Here we studied 30 congeneric ligands that each present a distinct heteroarene for stacking between tyrosine residues at the dimer interface of procaspase-6. Complex X-ray crystal structures of 10 analogs showed that stacking geometries were well conserved, while high-accuracy computations showed that heteroarene stacking energy was well correlated with predicted overall ligand binding energies. Here we employed a congeneric set of molecular glues for procaspase-6 to study diverse heteroarene stacking on tyrosine side chains under physiologically relevant conditions. As a model system, this protein–ligand interaction exhibits desirable features such as a shape-persistent binding site, a conserved ligand binding mode across diverse analogs, and the positioning of the probe heteroarene at the terminus of the ligand structure.

To confirm that binding poses and stacking interactions were conserved across analogs 1–30, we solved procaspase-6 complex crystal structures for 10 representative analogs spanning 3 orders of magnitude in measured KD value. Importantly, all 10 structures revealed binding poses almost exactly analogous to that adopted by 1, with the probe heterocycles positioned in apparently productive stacking interactions with tyrosine 198A and 198B. Also consistent with established guidance was the trend of increasing potencies from thiophene to furan, to pyrazole and imidazole (7 and 8) as well as the favorable effect of N-methylation of nitrogen-bearing heterocycles in the context of indazole (cf. 9 vs 15), imidazole (cf. 8 vs 18), and triazole (cf. 22 vs 24). Recently, Bootsma et al. noted the importance in heteroarene stacking of the relative positioning of ring heteroatoms in otherwise similar heterocycles. By contrast, the distal arrangement is favored when the heteroatoms are “dissimilar” (i.e., one is an amine-like nitrogen atom). We evaluated these predictions across the four relevant comparator sets, confining the analysis to analogs bearing an ortho N atom capable of IMHB formation. In the case of rings with dissimilar heteroatoms, we observe distal positioning to be favored, as predicted (cf. 7 and 8 vs 9 and 18 vs 15).

>MSSASGLRRGHPAGGEENMTETDAFYKREMFDPAEKYKMDHRRRGIALIFNHERFFWHLTLPERRGTCADRDNLTRRFSDLGFEVKCFNDLKAEELLLKIHEVSTVSHADADCFVCVFLSHGEGNHIYAYDAKIEIQTLTGLFKGDKCHSLVGKPKIFIIQAARGNQHDVPVIPLDVVDNQTEKLDTNITEVDAASVYTLPAGADFLMCYSVAEGYYSHRETVNGSWYIQDLCEMLGKYGSSLEFTELLTLVNRKVSQRRVDFCKDPSAIGKKQVPCFASMLTKKLHFFPKSNENLYFQ[4x]(Z)-docos-13-enoic acid | C22 H42 O2 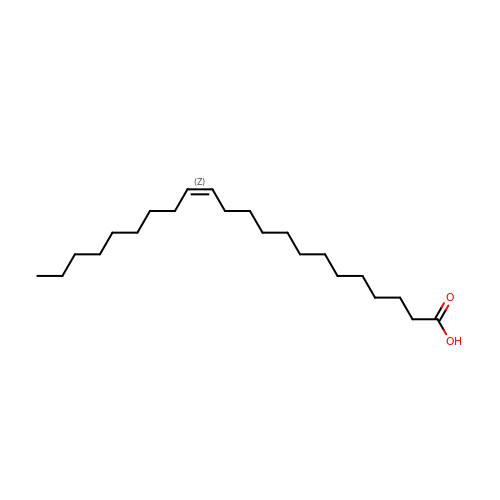| DPUOLQHDNGRHBS-KTKRTIGZSA-N>KGFSSEDKGEWKLKLDASGNGQAVIRFLPAKTDDALPFAILVNHGFKKNGKWYIETCSSTHGDYDSCPVCQYISKNDLYNTNKTEYSQLKRKTSYWANILVVKDPQAPDNEGKVFKYRFGKKIWDKINAMIAVDTEMGETPVDVTCPWEGANFVLKVKQVSGFSNYDESKFLNQSAIPNIDDESFQKELFEQMVDLSEMTSKDKFKSFEELNTKFNQVLGTA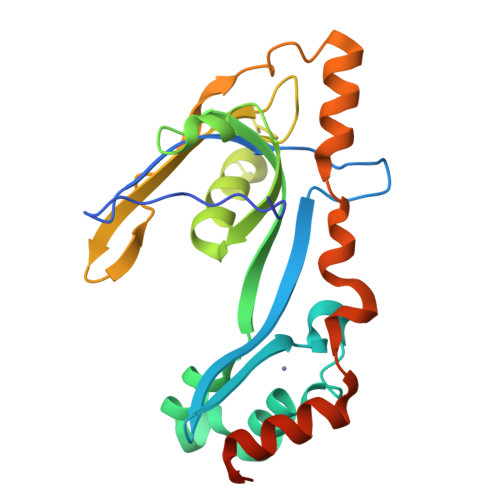ALGGAAAAAAS[2x]>MEQIAQQQPQTLCIKHLAKNYSKRWVVKDVSFEMQSGQIVGLLGPNGAGKTTSFYMVVGLVRMDKGEIHLDNLDLSDLAMHERARKGIGYLPQEASIFRKLTIAENIMAILETRKDLNKQQRQQRLQELLNDFKITHIKDSLGMSVSGGERRRAEIARALAADPKFMLLDEPFAGVDPISVGDIKDIIRNLKDRGIGVLITDHNVRETLAICEHAYIVSEGAVIAEGSPQDILENEQVRKVYLGDDFTV[2x];> MIIRRYLVKQVVSTSLVVIALLTLIMMGGRLIKYFGVAAQGRLDAGVLFSIIGYRMPEFLTLILPLGFFIGLMLVFGRLYVDHEMAVLNGSGISRIRLGQLLIPLALVFLVIQGILMLWMTPWGLRQFDQLSSSQAVRTGFDLVRPKEFISSGPYTIYAGDLSEDRKNLKDIFFYQRAQKEGKPDVMILAKEATRVVMENETANVVDLIQGRRYEIYPGKAKYSQAEFQRYRLRLENDKSATFETDKVEALPSSKLWNKWNDPVIASEMGWRVFGPFTIVIALMMAVALCEVSPRQGRYYRLIPAIFIFASLIVLLIAIRTRISRDELGVWAYPAALAVYGIAAALFSRKQKLAPKIKKQIKRVRA;> MLARRIVAKHVTKTTALAMLGTTIVLVILQVLFTYLGELSNLKADYSAWQAFLYVLWGAPRYLYEILPISALIGAILGLGTLASNSELIVMRSVGISLWRIVGWVIRSALVLVLLSFALSEWVVPYTNERANSVKSHQSVAALGEVRGYWSREGQRFIYVDYANSQGQLKRIQVVDFDDNYRLKSVTNAEQGQFVKDGQWLLNHSQQMAIQGQGDAVLANAAKQPFSLALQPKYVHMVTIDPEDLSFSQLVSFMNYMREYSQVPKTYQLAFWKKVASPFALITLVLVACSFIFGPLRQQSMGFRLVIALFIGLGFYYLQDFLGYASLVYNPSPAWFVLGPIVLMFVAGSYLLYRAR

The impenetrable nature of the outer membrane is due to the presence of a large, amphipathic glycolipid called lipopolysaccharide (LPS) in its outer leaflet. Assembly of the outer membrane requires transport of LPS across a protein bridge that spans from the cytoplasmic membrane to the cell surface. Here, using structural, biochemical and genetic approaches, we show that these antibiotics trap a substrate-bound conformation of the LPS transporter that stalls this machine. The inhibitors accomplish this by recognizing a composite binding site made up of both the Lpt transporter and its LPS substrate.

LptC also contains a TM helix that exists in two states. In one, the TM helix is sandwiched between the TM helices of LptG (helix 1) and LptF (helices 5 and 6), which form the gate through which LPS enters the transporter lumen. In a second state, the LptC helix has moved away from the transporter. Movement of the LptC helix between these states is thought to be important in coordinating LPS transport with the catalytic cycle of ATP binding and hydrolysis. We obtained a structure of A. baylyi LptB2FGC in the presence of LPS, although density for the LPS molecule was poorly resolved. Despite several attempts, we were unable to obtain an LptB2FGC complex in which 1 was also bound. These data are compatible with a model in which binding of 1 and binding of the TM helix of LptC at the LptFG gate are mutually exclusive. Superimposing the LptB2FG–LPS–1 structure with the LptB2FGC–LPS structure identified shifts in the conformation of LptFG, particularly in helices 4, 5 and 6 of LptF. This conformation of LptF creates a pocket between helices 4 and 5 that better accommodates acyl chain 6 of LPS.> MDQENFHGSSLPQQ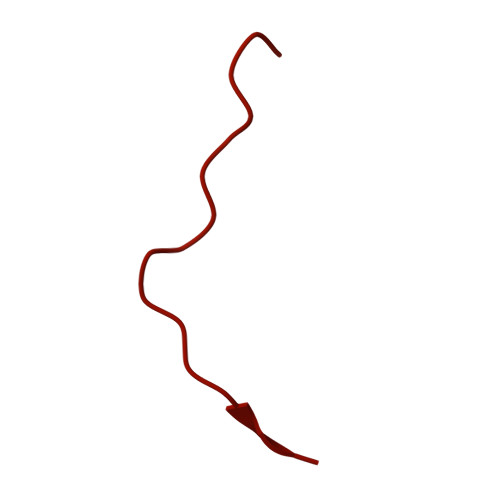LQNLHIQPQQASPNPVQTGFAPRRHYNNLVGLGNGNAVSGSPVKGAPLGQRHVKLKKEKISAQVAQLSQPGQLQLSDVGDPALAGGSGLQGGVGLMGVILPSDEALKFVSETDANGLAMKTPVSILQELLSRRGITPGYELVQIEGAIHEPTFRFRVSFKDKDTPFTAMGAGRSKKEAKHAAARALIDKLIGAQLPESPSSSAGPSVTGLTVAGSGGDGNANATGGGDASDKTVGNPIGWLQEMCMQRRWPPPSYETETEVGLPHERLFTIACSILNYREMGKGKSKKIAKRLAAHRMWMRLQETPIDSGKISDSICGELEGEVSIIQDIDRYEQVSKDFEFIKI>QSDSVSFTFPNFWSDVEDSIIFQGDANTTAGTLQLCKTNQYGTPLQWSAGRALYSDPVQLWDNKTESVASFYTEFTFFLKITGNGPADGLAFFL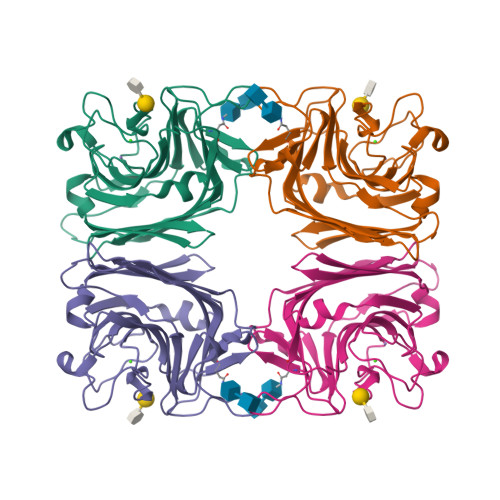APPDSDVKDAGEYLGLFNKSTATQPSKNQVVAVEFDTWTNPNFPEPSYRHIGINVNSIVSVATKRWEDSDIFSGKIATARISYDGSAEILTVVLSYPDGSDYILSHSVDMRQNLPESVRVGISASTGNNQFLTVYILSWRFSSNLQSTSVKAAMEPEITRTVV[2x]> MISTTISGKRPIEQVDDELLSLTAQQENEEQQQQRKRRRHQFAPMTQFNSNTLDEDSGFRSSSDVATADQDNFLEESPSGYIKKVILRNFMCHEHFELELGSRLNFIVGNNGSGKSAILTAITIGLGAKASETNRGSSLKDLIREGCYSAKIILHLDNSKYGAYQQGIFGNEIIVERIIKRDGPASFSLRSENGKEISNKKKDIQTVVDYFSVPVSNPMCFLSQDAARSFLTASTSQDKYSHFMKGTLLQEITENLLYASAIHDSAQENMALHLENLKSLKAEYEDAKKLLRELNQTSDLNERKMLLQAKSLWIDVAHNTDACKNLENEISGIQQKVDEVTEKIRNRQEKIERYTSDGTTIEAQIDAKVIYVNEKDSEHQNARELLRDVKSRFEKEKSNQAEAQSNIDQGRKKVDALNKTIAHLEEELTKEMGGDKDQMRQELEQLEKANEKLREVNNSLVVSLQDVKNEERDIQHERESELRTISRSIQNKKVELQNIAKGNDTFLMNFDRNMDRLLRTIEQRKNEFETPAIGPLGSLVTIRKGFEKWTRSIQRAISSSLNAFVVSNPKDNRLFRDIMRSCGIRSNIPIVTYCLSQFDYSKGRAHGNYPTIVDALEFSKPEIECLFVDLSRIERIVLIEDKNEARNFLQRNPVNVNMALSLRDRRSGFQLSGGYRLDTVTYQDKIRLKVNSSSDNGTQYLKDLIEQETKELQNIRDRYEEKLSEVRSRLKEIDGRLKSTKNEMRKTNFRMTELKMNVGKVVDTGILNSKINERKNQEQAIASYEAAKEELGLKIEQIAQEAQPIKEQYDSTKLALVEAQDELQQLKEDINSRQSKIQKYKDDTIYYEDKKKVYLENIKKIEVNVAALKEGIQRQIQNACAFCSKERIENVDLPDTQEEIKRELDKVSRMIQKAEKSLGLSQEEVIALFEKCRNKYKEGQKKYMEIDEALNRLHNSLKARDQNYKNAEKGTCFDADMDFRASLKVRKFSGNLSFIKDTKSLEIYILTTNDEKARNVDTLSGGEKSFSQMALLLATWKPMRSRIIALDQFDVFMDQVNRKIGTTLIVKKLKDIARTQTIIITPQDIGKIADIDSSGVSIHRMRDPERQNNSNFYN;> MGSVNSSPNEEFETVPDSQISGFDSPLIPTSVGSYFRDDDDDEKVHPNFISDPENDSLNSDEEFSSLENSDLNLSGAKAESGDDFDPILKRTIISKRKAPSNNEDEEIVKTPRKLVNYVPLKIFNLGDSFDDTITTTVAKLQDLKKEILDSPRSNKSIVITSNTVAKSELQKSIKFSGSIPEIYLDVVTKETISDKYKDWHFISKNCHYEQLMDLEMKDTAYSFLFGSSRSQGKVPEFVHLKCPSITNLLVLFGVNQEKCNSLKINYEKKENSRYDNLCTIFPVNKMLKFLMYFYSDDDNDDVREFFLKAFICLILDRKVFNAMESDHRLCFKVLELFNEAHFINSYFEIVDKNDFFLHYRLLQIFPHLQSALLRRRFSEKQGRTETIQQNIIKEFNEFFDCKNYKNLLYFILTMYGSKFIPFGPKCQVTEYFKDCILDISNETTNDVEISILKGILNLFSKIR;> MDGALINSVLYVSPRNGAHYFVELTEKHLLAFEMLNSMCLLENYDHVLLFLECQFGKSHNLAVIPFDIILVLFTLSTLSEYYKEPILRANDPYNTSRETLSRRALKLLQKYLAILKEFDSEQYNLYDLELLRCQFFLAIDTLTPKKQKWGFDRFRRTKSESGVTYRQNASVDPELDQAKTFKNPYRSYISCLEQRNTILGNRLLNLKLNEPGEFINMILWTLSNSLQESTPLFLSSHEIWMPLLEILIDLFSCRQDYFIQHEVAQNVSKSLFVQRLSESPLAVFFESLNTRNFANRFSEYVFLNCDYKLPSDNYATPVHPVYNGENTIVDTYIPTIKCSPLYKSQKSLALRRKLIG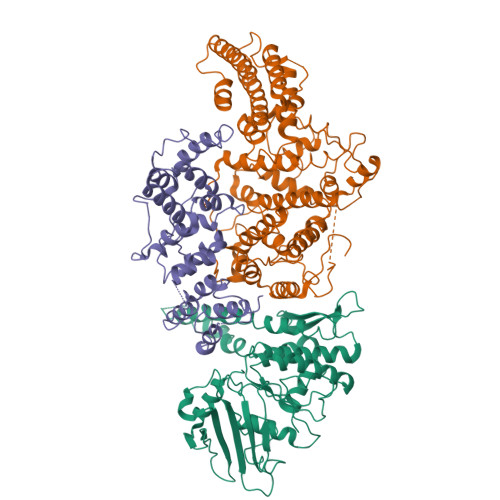SCFKLLLRVPDGHRLITPRIVADDVIQGISRTLASFNDILQFKKFFMTENLSQESYFIPLLAEGTLSEILKDTQECVVILTLVENLSDGVSFCNEVIGLVKSKCFAFTEQCSQASYEEAVLNIEKCDVCLLVLLRYLLHLIGTEAILDAKEQLEMLHAIEKNDSGRRQWAKALNLGNDPPLLYPIVSQMFGVHDKSVIIE>MNTIAWLGRLVIERIRGIGVAALMLLQIIFSLPSAGGFGRFVYQMHRVGVMSLLIITVSGLFIGLVLGLQGYSILVNVGSESMLGTMVSLTLLRELAPVVAALLFAGRAGSALTAEIGSMKQSEQLASMEMIGVDPLKQIVSPRLWAGIVSLPMLTVIFAAIGIVGGKLVGVDFLGVDEGSFWSGMQNNVQFGHDVVNGIIKSIVFALLCTWIAVFQGYACDPTPEGIATAMTRTVVYSSLCVLGFDFVLTAVMFGGI[2x];>MMNNKTPLSTQSLIEVKNLSFNRGERVIYDNISLNIRRGQITAIMGPSGTGKTTLLRLIGGQLVPDQGEVLLDGKDIAQMSRQELFAARARMGMLFQSGALFTDMSVYENVAFPIRAHTKLSENLIAELVALKLESVGLRGTEQLMPTELSGGMNRRVALARAIALDPDLIMYDEPFAGQDPIVKGVLTRLIRSLREALDLTTIIVSHDVPETLSIADYIYVVAEGKIQGEGTPEELQAYASPFVKQFLTGSAEGPVEYQFSHQAYLDNEVRP[2x];>[2x]VVQYLNQELVVSGKIDFENAEQQYQAGLAIIKKQTSFPLIVDLKQLEHGNTLALAVLVQWLRQTPQKSGLHFKNVPEKMLKIIQACHLQEDLHLVLEHHHHHH;>MKSRTSELAVGIFVIIFGIALFFLAMKVSGLVGTNLSDGYTMKAQFDNVNGLKPRAKVTMSGVTIGRVDSITLDPVTRLATVTFDLDGKLTSFNAEQLKEVQKNALDELRYSSDYTQATPAQQKTMEQQLISNMNSITSIDEDAYIMVATNGLLGEKYLKIVPGGGLNYLKRGDTISNTQGTMDLEDLISKFITGGGAGKVAAGSSSAEEKAPASTDSSAQPSFVE[6x]

The MlaFEDB complex is an ATP-binding cassette transporter to actively translocate the phospholipids between the inner membrane and the periplasmic protein MlaC4,5. The MlaFEDB-mediated glycerophospholipid (PL) transport was reported to play an important role in maintaining the integrity of the lipid membrane. Consistent with the previous reported low-resolution A. baumannii MlaFEDB map8 and our E. coli MlaFEDB map9 (EMD-30355), the MlaF (cytoplasmic nucleotide-binding domain, NBD), MlaE (transmembrane domain), MlaD (periplasmic phospholipid-binding domain), and MlaB (cytoplasmic auxiliary domain) subunits are assembled in a stoichiometry of 2:2:6:2. In summary, we characterize four structures of the A. baumannii MlaFEDB complex in nucleotide-free and vanadate-trapped conformations using single-particle cryo-EM.

To understand the mechanism of glycerophospholipid translocation coupled with the conformational change, distinct conformations of MlaFEDB were trapped using sodium ortho-vanadate. Vanadate acts as a potent inhibitor of ATPase by forming an ADP–vanadate complex that mimics the intermediate state formed during hydrolysis. Three individual conformations were classified and refined to 4.0, 3.6, and 4.0 Å, and were named Vtrans1, Vtrans2, and Vclose, respectively. The structure of Vclose shows the tight dimerization and close proximity of the NBD of MlaF subunits, caused by the trapping of ADP–vanadate or ATP at the ATP-binding sites comprising the Walker A, Walker B motifs, and the signature motif. The dimerization of the NBDs engages the coupled structural rearrangements of MlaE and MlaD, respectively. The MlaD ring rotates clockwise and the two subunits of MlaE squeeze towards each other to collapse the central phospholipid-binding cavity to extrude lipids. No bound glycerophospholipid densities were observed in the central cavity in Vclose. All three structures display bound nucleotides at the ATP-binding sites. However, the maps are of insufficient quality to distinguish between ADP, ATP, and ADP–vanadate. The three vanadate-trapped structures of MlaFEDB reveal different levels of conformational rearrangement of MlaD and MlaE coupled with nucleotide binding and glycerophospholipid translocation.>[2x]MHYSNIEANESEEERQFRKLFVQLAGDDMEVSATELMNILNKVVTRHPDLKTDGFGIDTSRSMVAVMDSDTTGKLGFEEFKYLWNNIKKWQGIYKRFD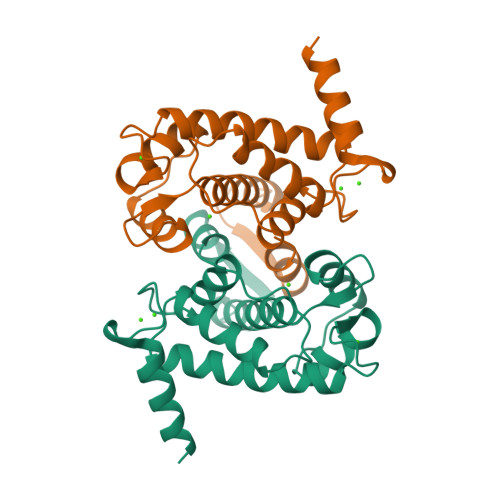TDRSGTIGSNELPGAFEAAGFHLNQHIYSMIIRRYSDETGNMDFDNFISCLVRLDAMFRAFRSLDKNGTGQIQVNIQEWLQLTMYS>[2x]GSFTMEPLKVEKFATANRGNGLRAVTPLRPGELLFRSDPLAYTVCKGSRGVVCDRCLLGKEKLMRCSQCRVAKYCSAKCQKKAWPDHKRECKCLKSCKPRYPPDSVRLLGRVVFKLMDGAPSESEKLYSFYDLESNINKLTEDKKEGLRQLVMTFQHFMREEIQDASQLPP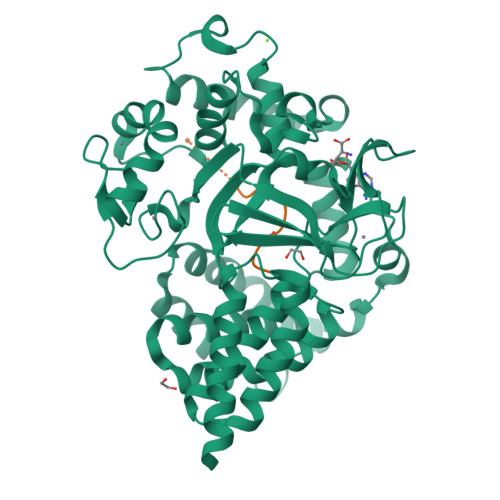AFDLFEAFAKVICNSFTICNAEMQEVGVGLYPSISLLNHSCDPNCSIVFNGPHLLLRAVRDIEVGEELTICYLDMLMTSEERRKQLRDQYCFECDCFRCQTQDKDADMLTGDEQVWKEVQESLKKIEELKAHWKWEQVLAMCQAIISSNSERLPDINIYQLKVLDCAMDACINLGLLEEALFYGTRTMEPYRIFFPGSHPVRGVQVMKVGKLQLHQGMFPQAMKNLRLAFDIMRVTHGREHSLIEDLILLLEECDANIRAS;>YDNPIFEKFGKGGTYX[2x]> AVSKGFNYGATKADGSSKYQADFKKDFAAAKALVEGGSGFTSARLYTMIQGGTTNTPIEAIPAAIEEKTELLLGLWASGGNMDNEIAALKSAISQYGDDFANLVVGISVGSEDMYRNSVTGSKSNAGPGVEPEELVSYIQQVRSTIAGTGLSDASIGHVDTWDSWTNSSNSDVVNHLDWLGFDGYPYYQLTMENGIENAKKLFDESVEKTKSVANGKEVWITETGWPVTGPQEGDATASPANAKTYWDEVGCPLFGNTNTWWYMLEDEGASPSFGVVKSDLKTPQFDLSC

To provide new insight into the glucan metabolism in the Penicillium genus, we focused on two enzymes (named G9376 and G7048) that have been previously identified in the culture filtrate of P. sumatraense AQ67100 fed with C. vulgaris biomass. On the other hand, in contrast to its predicted function, G7048 acts as a 1,3-β-transglucanase active on 1,3-β-glucan oligomers with a degree of polymerization (DP) higher than 5. Enzymatic analyses revealed that G7048 acts as a 1,3-β-transglucanase, rather than a glucanase as inferred by predictions, creating branched-glucans. The antagonizing activity between G9376 and G7048 suggests how opportunistic species belonging to Penicillium genus may feed on substrates with a composition similar to their own cell wall without incurring in self-deleterious autohydrolysis.

Moreover, since this region has been predicted to bind a glycosylphosphatidylinositol (GPI) tail for the anchoring of G7048 to the cell membrane, we decided to express a truncated variant of the protein encompassing the first 308 residues (hereafter referred to as ΔG7048). The X-ray crystallographic structure of the catalytic domain of G7048, solved at 1.9 Å of resolution, consists of a (β/α)8 TIM-barrel fold characteristic of all the GH17 family members. The catalytic site is in a V-shaped cleft containing the two conserved catalytic glutamic residues. An important feature of ΔG7048 is the absence of the so-called “subdomain” in the proximity of the helix α6, which is present in other glycoside hydrolase of the GH17 family and has been proposed to provide subsites + 3, + 4 and + 5 for substrate binding in 1,3-β-glucanase. Notably, ΔG7048 shares this peculiar feature with RmBgt17A, a protein belonging to the GH17 family, which acts as a β-1,3-glucanosyltransferase. Moreover, albeit ΔG7048 and RmBgt17A share a low amino acid identity (29%), both the catalytic glutamic residues (E111 and E222) and several aromatic residues pointed out by Qin and colleagues as involved in direct substrate binding in RmBgt17A are conserved or conservatively mutated in ΔG7048. Structural and mutagenesis studies have identified three of these residues (Y102, W157, and E158 in RmBgt17A) as crucial for transglycosylation activity toward hydrolytic activity. In the ΔG7048 structure, their topological position is occupied by the residues Y114 (Y102), Y187 (W157), and Q188 (E158) which are likely to fulfill the same proposed role in the stabilization of the transition state at subsite − 1, + 1 and + 2 during the transglycosylation reaction step. In the ΔG7048 structure, their topological position is occupied by W161, D162, Q188 and S205 which, together with the structural elements in regions 2 and 3 are likely to create a similar steric hindrance.> VVSLDKPFMYFEEIDNELDYEPESANEVAKKLPYQGQLKLLLGELFFLSKLQRHGILDGATVVYIGSAPGTHIRYLRDHFYNLGVIIKWMLIDGRHHDPILNGLRDVTLVTRFVDEEYLRSIKKQLHPSKIILISDVRSKRGGNEPSTADLLSNYALQNVMISILNPVASSLKWRCPFPDQWIKDFYIPHGNKMLQPFAPSYSAEMRLLSI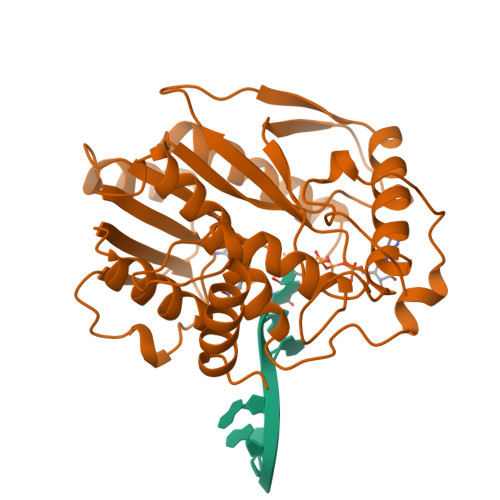YTGENMRLTRVTKSDAVNYEKKMYYLNKIVRNKVVVNFDYPNQEYDYFHMYFMLRTVYCNKTFPTTKAKVLFLQQSIFRFLNIP> MNKLVGLLVSSLFLASILIGIAPAITTTALTPPVSAGGIQAYLLTGSGAPASGLVLFVVNVSNIQVSSSNVTNVISTVVSNIQINAKTENAQTGATTGSVTVRFPTSGYNAYYDSVDKVVFVVVSFLYPYTTTSVNIPLSYLSKYLPGLLTAQPYDETGAQVTSVSSTPFGSLIDTSTGQQILGTNPVLTSYNSYTTQANTNMQEGVVSGTLTSFTLGGQSFSGSTVPVILYAPFIFSNSPYQAGLYNPMQVNGNLGSLSSEAYYHPVIWGRALINTTLIDTYASGSVPFTFQLNYSVPGPLTINMAQLAWIASINNLPTSFTYLSYKFSNGYESFLGIISNSTQLTAGALTINPSGNFTINGKKFYVYLLVVGSTNSTTPVEYVTKLVVEYPSSTNFLPQGVTVTTSSNKYTLPVYEIGGPAGTTITLTGNWYSTPYTVQITVGSTPTLTNYVSQILLKAVAYEGINVSTTQSPYYSTAILSTPPSEISITGSSTITAQGKLTATSASATVNLLTNATLTYENIPLTQYSFNGIIVTPGYAAINGTTAMAYVIGALYNKTSDYVLSFAGSQEPMQVMNNNLTEVTTLAPFGLTLLAPSVPATETGTSPLQLEFFTVPSTSYIALVDFGLWGNLTSVTVSAYDTVNNKLSVNLGYFYGIVIPPSISTAPYNYQNFICPNNYVTVTIYDPDAVLDPYPSGSFTTSSLPLKYGNMNITGAVIFPGSSVYNPSGVFGYSNFNKGAAVTTFTYTAQSGPFSPVALTGNTNYLSQYADNNPTDNYYFIQTVNGMPVLMGGLSIVASPVSASLPSSTSSPGFMYLLPSAAQVPSPLPGMATPNYNLNIYITYKIDGATVGNNMINGLYVASQNTLIYVVPNGSFVGSNIKLTYTTTDYAVLHYFYSTGQYKVFKTVSVPNVTANLYFPSSTTPLYQLSVPLYLSEPYYGSPLPTYIGLGTNGTSLWNSPNYVLFGVSAVQQYLGFIKSISVTLSNGTTVVIPLTTSNMQTLFPQLVGQELQACNGTFQFGISITGLEKLLNLNVQQLNNSILSVTYHDYVTGETLTATTKLVALSTLSLVAKGAGVVEFLLTAYPYTGNITFAPPWFIAENVVKQPFMTYSDLQFAKTNPSAILSLSTVNITVVGLGGKASVYYNSTSGQTVITNIYGQTVATLSGNVLPTLTELAAGNGTFTGSLQFTIVPNNTVVQIPSSLTKTSFAVYTNGSLAIVLNGKAYSLGPAGLFLLPFVTYTGSAIGANATAIITV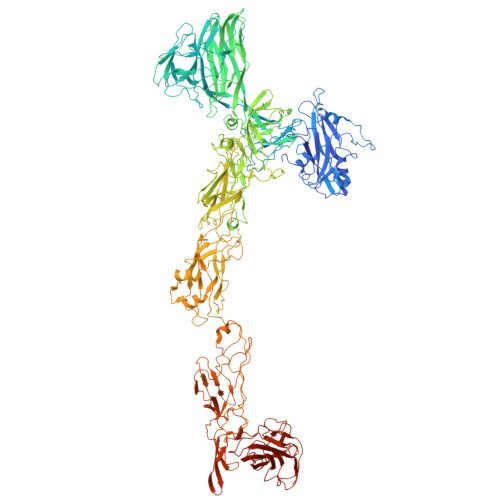SDGVGTSTTQVPITAENFTPIRLAPFQVPAQVPLPNAPKLKYEYNGSIVITPQQQVLKIYVTSILPYPQEFQIQAFVYEASQFNVHTGSPTAAPVYFSYSAVRAYPALGIGTSVPNLLVYVQLQGISNLPAGKYVIVLSAVPFAGGPVLSEYPAQLIFTNVTLTQ N~4~,N~6~-dicyclopentyl-2-(methylsulfanyl)-5-nitropyrimidine-4,6-diamine | C15 H23 N5 O2 S | 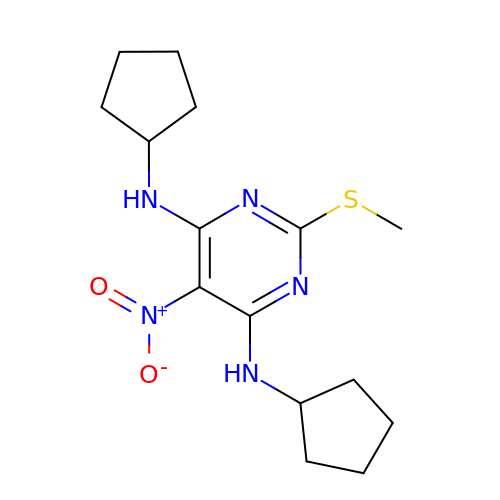GSGVDKOCBKBMGG-UHFFFAOYSA-N>[4x]GFEERSGVVPCGTPWGQWYQTLEEVFIEVQVPPGTRAQDIQCGLQSRHVALAVGGREILKGKLFDSTIADEGTWTLEDRKMVRIVLTKTKRDAANCWTSLLESEYAADPW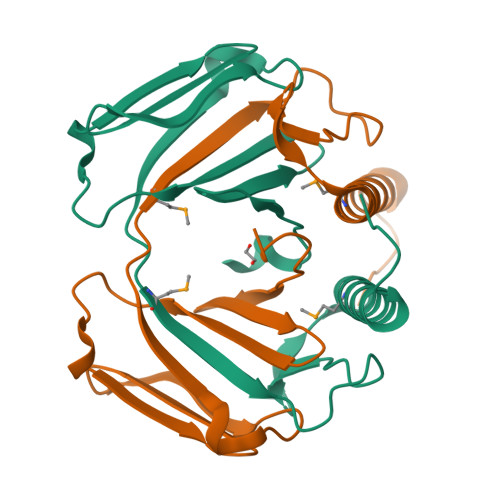VQDQMQRKLTLERFQKENPGFDFSGAEISGNYTKGGPDFSNLGNDGT> GSLPAHSLVMSSPALPAFLLCSTLLVIKMYVVAIITGQVRLRKKAFANPEDALRHGGPQYCRSDPDVERCLRAHRNDMETIYPFLFLGFVYSFLGPNPFVAWMHFLVFLVGRVAHTVAYLGKLRAPIRSVTYTLAQL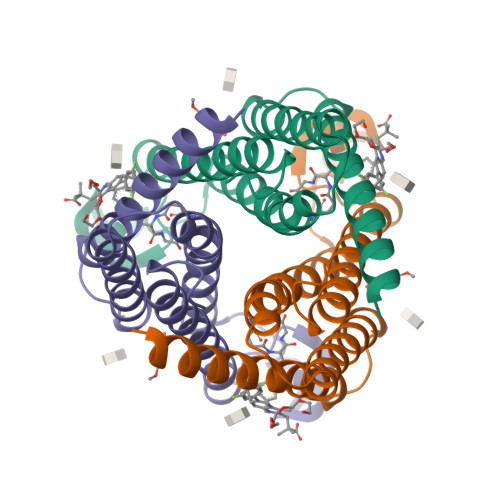PCASMALQILWEAARHL> AFPDCANGPLKSNLVCNASADPVSRA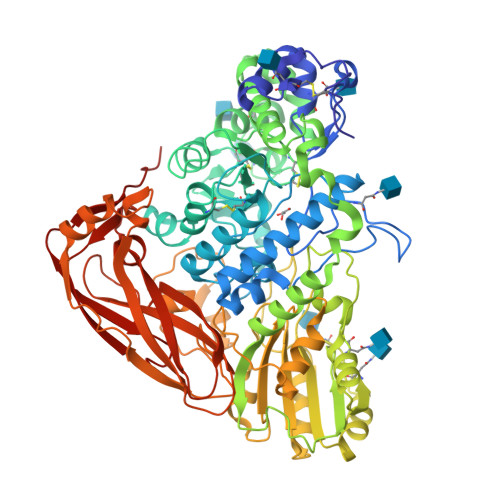KALVDALTLEELVNNTVNASPGVPRVGLPPYNWWSEALHGVARSPGANFSTVPGSPFSSATSFPQPIILGATFDDDLIHSIATVISTEARAFNNAGRAGLDFFTPNINPFKDPRWGRGQETPGEDPYHIAQYVYQLITGLQGGLSPDPYYKVVADCKHFAGYDLEDWHGNNRMAFNAVISTQDLAEFYTPSFQSCVRDAHVGSVMCSYNAVNGVPSCASPYLLQDLIRDHFGLGDGWITSDCDAVDNVFDPHNYTSTLVNASAVSLKAGTDVDCGTTYSQTLVDAVNQKLVTEDDVKTSMVRLYSSLVRLGYFDSPENQPWRQLGWADVNTPSAQALALTAAEEGVVLLKNDGTLPLSRRIKHIAVVGPWANATTQMQGNYQGIAPFLISPLQALQDAGFHVSFANGTAINSTDTSGFASALMAAKAADAIVFAGGIDETIESEGHDRDSIEWPGNQLDLIEQLAALRKPLIVLQMGGGQVDSSSLKASKAVNALLWGGYPGQSGGTAIVNILTGKTAPSGRLPITQYPAAYVDAIPMTDMALRPSSSSPGRTYKWYTGTPVFDFGFGLHYTSFKLSWAASPPSRFDISSLVAGAKHAGVAFTDLAPLFTFHVAVKNSGKVTSDYVALLFAHTTVGPSPAPQQELVAYTRVKGITPGRTATAALSVTLGSIARVDESGVRSLYPGKYSVWVDTTREIMHTFELTGKTTQILGWPQPR> MELQPQFNEFLANIRPTDTQKEDWKSGARTLRERLKNFEPLKEIVVSTFLQGSI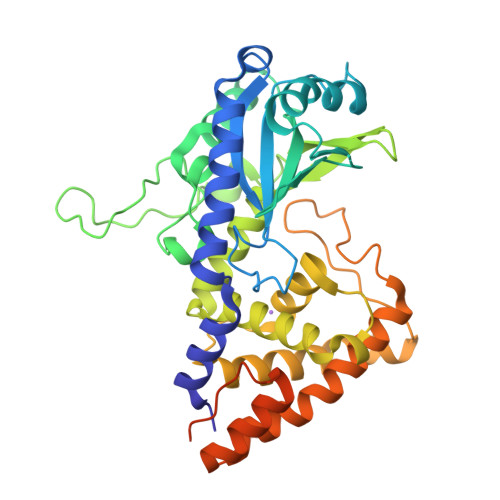RRSTAIRPLGDKRPDVDIVVVTNLDHTRMSPTDAMDLFIPFLEKYYPGKWETQGRSFGITLSYVELDLVITAIPESGAEKSHLEQLYKSESVLTVNSLEEQTDWRLNKSWTPNTGWLSESNSAQVEDAPASEWKAHPLVLPDREKNEWGRTHPLAQIRWTAEKNRLCNGHYINLVRAVKWWRQQNSEDLPKYPKGYPLEHLIGNALDNGTTSMAQGLVQLMDTFLSRWAAIYNQKSKPWLSDHGVAEHDVMARLTAEDFCSFYEGIASAAEIARNALASEEPQESAQLWRQLFGSKFPLPGPQGGDRNGGFTTPSKPAEPQKTGRFALEHHHHHH>[2x]MGKRVLIVDDAAFMRMMLKDIITKAGYEVAGEATNGRE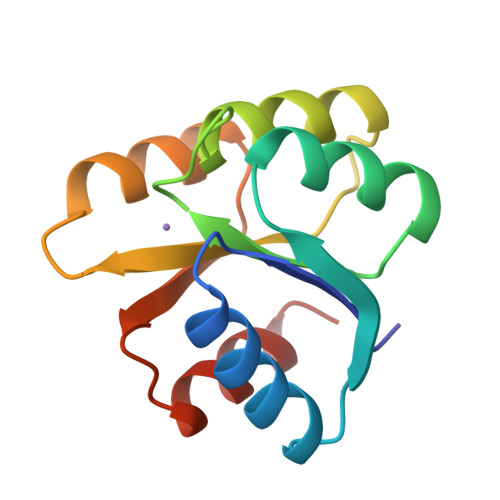AVEKYKELKPDIVTMDITMPEMNGIDAIKEIMKIDPNAKIIVCSAMGQQAMVIEAIKAGAKDFIVKPFQPSRVVEALNKVSK(2~{S})-~{N}-(5-methyl-6-oxidanylidene-benzo[b][1,4]benzothiazepin-2-yl)oxolane-2-carboxamide | 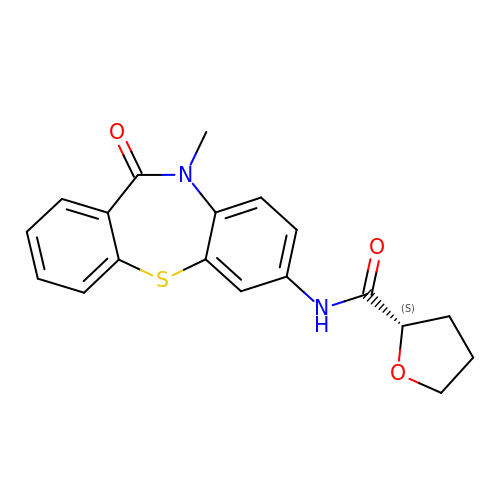C19 H18 N2 O3 S | DOZUHRRHXYFZFW-HNNXBMFYSA-N> APDIPLANVKAHLTQLSTIAANNGGNRAHG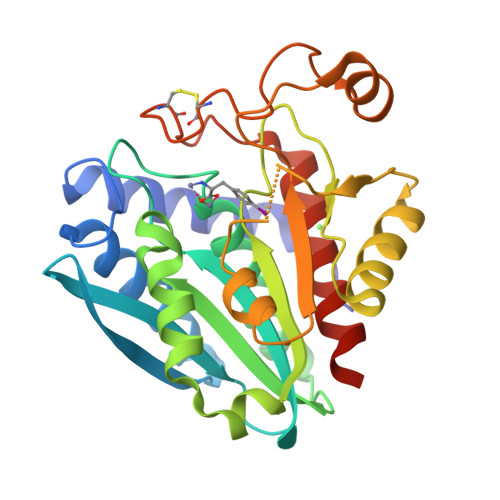RPGYKASVDYVKAKLDAAGYTTTLQQFTSGGATGYNLIANWPGGDPNKVLMAGAHLDSVSSGAGINDNGSGSAAVLETALAVSRAGYQPDKHLRFAWWGAEELGLIGSKFYVNNLPSADRSKLAGYLNFDMIGSPNPGYFVYDDDPVIEKTFKNYFAGLNVPTEIETEGDGRSDHAPFKNVGVPVGGLFTGAGYTKSAAQAQKWGGTAGQAFDRCYHSSCDSLSNINDTALDRNSDAAAHAIWTLSSGTGEPPT>[2x]GPLGSPVVVRGWLHKQDSSGMRLWKRRWFVLADYCLFYYKDSREEAVLGSIPLPSYVISPVAPEDRISRKYSFKAVHTGMRAL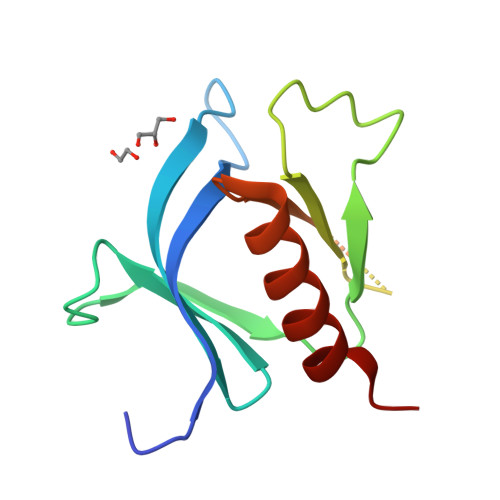IYNSSTAGSQAEQSGMRTYYFSADTQEDMNAWVRAMNQAAQVLS>SNATNNLEKELLDNFKKNITQYAKQLEISIEKVYDEKGSVNAQKDIQNLLSEYANMQEIGEIRFIDKDQIIIATTKQSNRSLINQKANDSSVQKALSLGQSNDHLILKDYGGGKDRVWVYNIPVKVDKKVIGN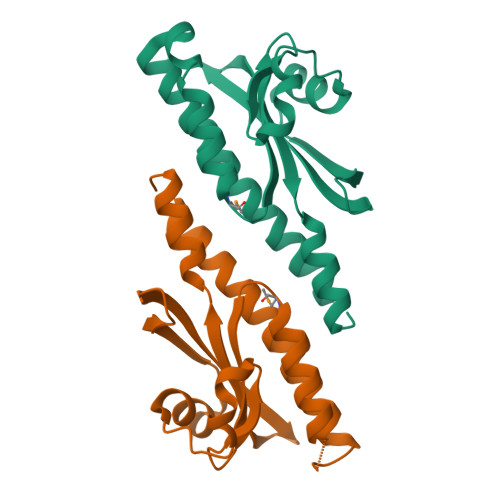IYIESKINDVYNQLNNINQ[2x]>MFKDGSLIPY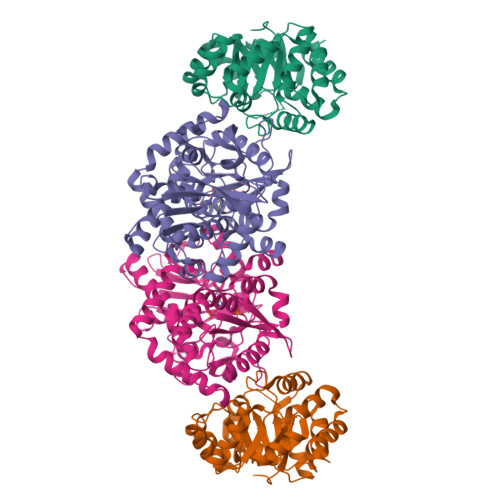LTAGDPDKQSTLNFLLALDEYAGAIELGIPFSDPIADGKTIQESHYRALKNGFKLREAFWIVKEFRRHSSTPIVLMTYYNPIYRAGVRNFLAEAKASGVDGILVVDLPVFHAKEFTEIAREEGIKTVFLAAPNTPDERLKVIDDMTTGFVYLVSLYGTTGAREEIPKTAYDLLRRAKRICRNKVAVGFGVSKREHVVSLLKEGANGVVVGSALVKIIGEKGREATEFLKKKVEELLGI[6x];>MWFGEFGGQYVPETLIEPLKELEKAYKRFKDDEEFNRQLNYYLKTWAGRPTPLYYAKRLTEKIGGAKIYLKREDLVHGGAHKTNNAIGQALLAKFMGKTRLIAETGAGQHGVATAMAGALLGMKVDIYMGAEDVERQKMNVFRMKLLGANVIPVNSGSRTLKDAINEALRDWVATFEYTHYLIGSVVGPHPYPTIVRDFQSVIGREAKAQILEAEGQLPDVIVACVGGGSNAMGIFYPFVNDKKVKLVGVEAGGKGLESGKHSASLNAGQVGVFHGMLSYFLQDEEGQIKPTHSIAPGLDYPGVGPEHAYLKKIQRAEYVTVTDEEALKAFHELSRTEGIIPALESAHAVAYAMKLAKEMSRDEIIIVNLSGRGDKDLDIVLKVSGNVLEHHHHHH[6x]> GAMAGKAVPMQSKKKIFKPEELRQALMPTLEALYRQDPESLPFRQPVDPQLLGIPDYFDIVKSPMDLSTIKRKLDTGQYQEPWQYVDDIWLMFNNAWLYNRKTSRVYKYCSKLSEVFEQEIDPVMQSLGYCCGRKLEFSPQTLCCYGKQLCTIPRDATYYSYQNRYHFCEKCFNEIQGESVSLGDDPSQPQTTINKEQFSKRKNDTLDPE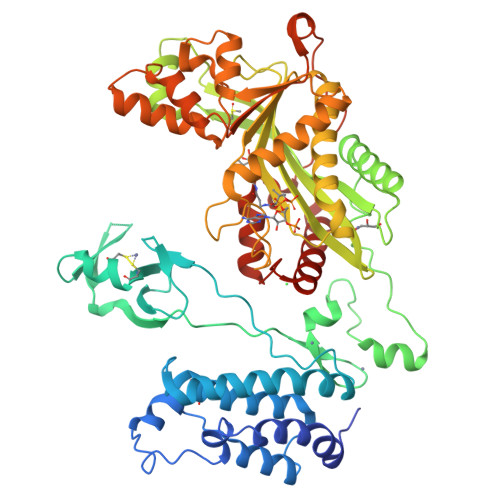LFVECTECGRKMHQICVLHHEIIWPAGFVCDGCLKKSARTRKENKFSAKRLPSTRLGTFLENRVNDFLRRQNHPESGEVTVRVVHASDKTVEVKPGMKARFVDSGEMAESFPYRTKALFAFEEIDGVDLCFFGMHVQEYGSDCPPPNQRRVYISYLDSVHFFRPKCLRTAVYHEILIGYLEYVKKLGYTTGHIWACPPSEGDDYIFHCHPPDQKIPKPKRLQEWFKKMLDKAVSERIVHDYKDIFKQATEDRLTSAKELPYFEGDFWPNVLEESIKESGGSGSQKLYATMEKHKEVFFVIRLIAGPAANSLPPIVDPDPLIPCDLMDGRDAFLTLARDKHLEFSSLRRAQWSTMCMLVELHTQSQDRF> MQAASAFATCLLASVGGNSSAVAFPNQANYSTLVAPYNFDLLTTPSAIVWPQDTQQVAAAVKCAVDSDIKVQPKSGGHNYGNYGSTTGELSVNLDNLQHFSMNETSWTARLGPGNRLGRVTELMYNNGGRHVPHGTTFTVGLGGHATVGGAGAASRMHGLLLDYVEEVEVVLANSSIVRASKSHNEDLFFAVRGAASSVGIVTDFSIRTEPVPVSSVTYSYIWEGTDPAARAEVFLTWQSLLAGGSLPQHMAYDLVATANSMILGGAYFGSQEDFEAFNLSSHFKVAPDVTHIKTYTNFFDFSAAASAQTKAAGIASPSHFYAKSLVFNQQTLIPDDAAEEVFKYLATTKNGTDLYAVTFAALGGAVRDVSASETAFYHRDASYFMFSFGRTSGDLTDTTVQFLDGLSEVLTSGQPDAYYGQYVGNVDPRQPTDEALTGYYGKNLHRLQQIKSAVDPNDVFHNQQSIPPLS

Sorbicillinoids are yellow secondary metabolites synthesized through an elegant combination of enzymatic and spontaneous biochemical processes. The flavin-dependent monooxygenase SorC and oxidase SorD are crucial in this interplay, enabling the generation of a diverse array of functionally complex sorbicillinoids. SorA and SorB work in tandem to synthesize the hexaketide precursor sorbicillin, while SorC and SorD are involved in the subsequent oxidative processes, including dimerization and oxidation reactions.11,12 Specifically, the monooxygenase SorC catalyzes the oxidative dearomatization of sorbicillin to form (S)-sorbicillinol. The oxidase SorD can then use hydrated sorbicillinol and oxidize it to oxosorbicillinol.

The C-terminally His6-tagged SorD from Penicillium chrysogenum ATCC 48,271 was produced in Aspergillus niger following a CRISPR/Cas9-based expression method. SorD crystallized as a monomer, consistent with size-exclusion chromatography and mass photometry. SorD belongs to the vanillyl-alcohol oxidase/p-cresol methylhydroxylase (VAO/PCMH) family and more specifically to the berberine bridge enzyme (BBE) subfamily. As with other oxidases from the VAO/PCMH family, the general structure of SorD contains two domains (1.55 Å): the N-terminal FAD domain (residues 45–212) and the C-terminal substrate-binding domain (residues 213–435). SorD also comprises a short C-terminal BBE domain (residues 436–468). The structure contains the partial remains of the N-terminal signal peptide (residues 5–22), and five N-glycosylation sites were identified (Asn18, Asn29, Asn174, Asn279, and Asn351). Several members of the BBE subfamily are characterized by (bi)covalent incorporation of the flavin cofactor. This feature was also found in SorD, where the FAD is covalently attached to residue His78. Covalent tethering of the flavin cofactor in BBE-like oxidases allows for a rather open active site that facilitates the entry of such bulky substrates. Moreover, upon testing the thermostability of SorD, we found that the enzyme is more stable under acidic conditions, with the highest melting temperature of 66 °C observed at pH 4.5.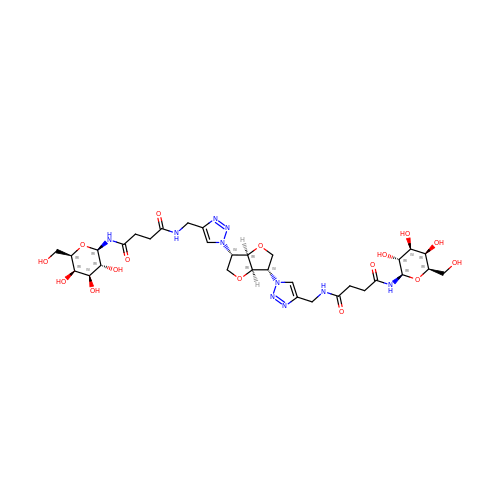N-[[1-[(3S,3aR,6S,6aR)-6-[4-[[[4-[[(2R,3R,4S,5R,6R)-6-(hydroxymethyl)-3,4,5-tris(oxidanyl)oxan-2-yl]amino]-4-oxidanylidene-butanoyl]amino]methyl]-1,2,3-triazol-1-yl]-2,3,3a,5,6,6a-hexahydrofuro[3,2-b]furan-3-yl]-1,2,3-triazol-4-yl]methyl]-N'-[(2R,3R,4S,5R,6R)-6-(hydroxymethyl)-3,4,5-tris(oxidanyl)oxan-2-yl]butanediamide | C32 H48 N10 O16 | WUNJKQMXDITVGU-ADJUJXGJSA-N4-(4-bromophenyl)-1H-imidazole | C9 H7 Br N2 | 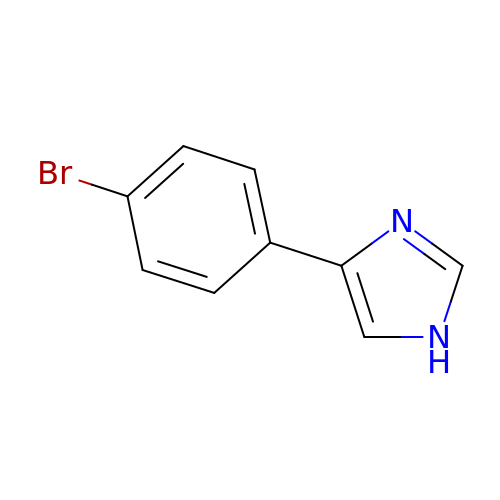YLIOAWKNPLJMID-UHFFFAOYSA-N>EEYSSNWAGAVLIGDGYTKVTGEFTVPSVSAGSSGSSGY[2x];>QSEEYCASAWVGIDGDTCETAILQTGVDFCYEDGQTSYDAWYEWYPDYAYDFSDITISEGDSIKVTVEATSKSSGSATVENLTTGQSVTHTFSGNVEGDLCETNAEWIVEDFESGDSLVAFADFGSVTFTNAEATSGGSTVGPSD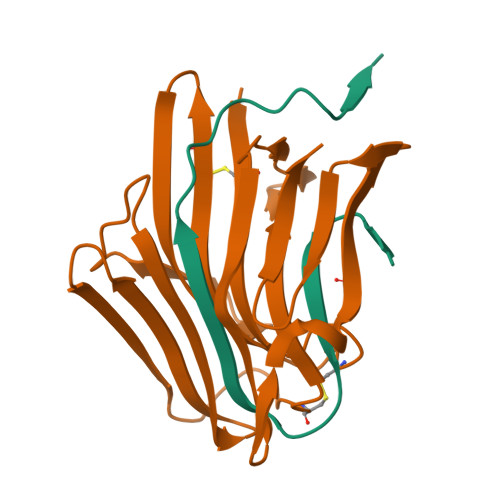ATVMDIEQDGSVLTETSVSGDSVTVTYV[2x]> GMFNESDAPQPPKVLSTPLEIAANLRQLQESHDPLIITFHDRSHRFQSYVVHVDRESNTLALDEMIPRDGEKFIENGEHFRVEGFHDGVRIAWECDHALKISEVDGHRCYSGPLPQEVTYHQRRNAFRAALKLSQLVDIILDGAHLKGNGAMRGKLLDISATGCKLRFEGNVEDRLQLGQVY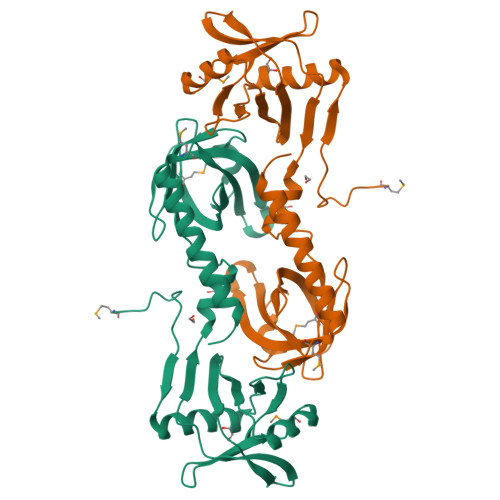ERFKAGNPLGLVDTMVELRHLHYEERINTTFAGVRFHNLSGQAQRKIESFVYQLQREARRFDKDDY1-CIS-9-OCTADECANOYL-2-CIS-9-HEXADECANOYL PHOSPHATIDYL GLYCEROL 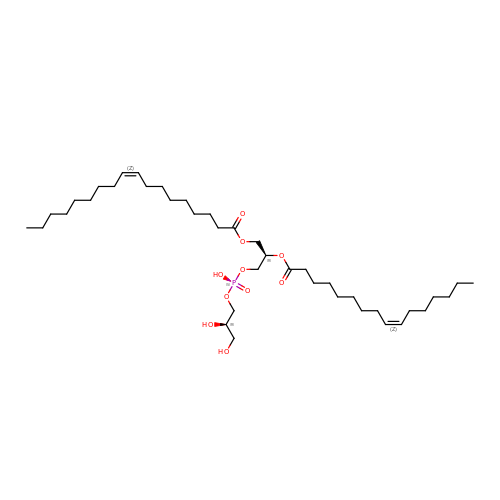| C40 H75 O10 P | QGIXWNRQEFVVRM-CTDKCSBDSA-N>[60x]MRRKVKNTKRHQWRLTHSARSIKRANIMPSNPRGGRRF;>[60x]MKKKMSKLNARVHDFSMFKGNHIPRSKIHIPHKTIRAFNVGEIIPIYQTPVYPGEHIKMDLTSLYRPSTFIVPPMDDLIVDTYAFAVPWRIVWKDLEKFFGENSDSWD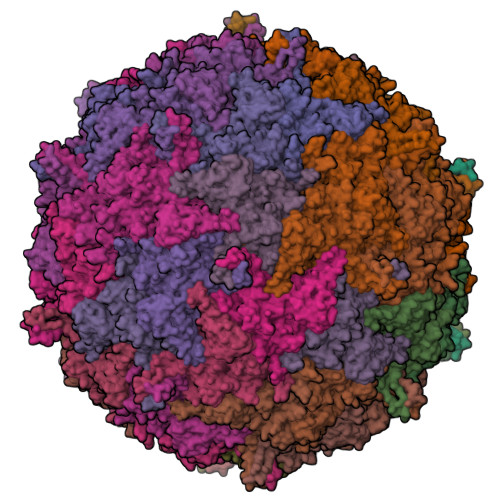VKNAPPVPDIVAPSGGWDYGTLADHFGITPKVPGIRVKSLRFRAYAKIINDWFRDQNLSSECALTLDSSNSQGSNGSNQVTDIQLGGKPYIANKYHDYFTSCLPAPQKGAPTTLNVGGMAPVTTKFRDVPNLSGTPLIFRDNKGRTIKTGQLGIGPVDAGFLVAQNTAQAANGERAIPSNLWADLSNATGISISDLRLAITYQHYKEMDARGGTRYVEFTLNHFGVHTADARLQRSEFLGGHSQSLLVQSVPQTSSTVEKMTPQGNLAAFSETMIQNNYLVNKTFTEHSYIIVLAVVRYKHTYQQGIEADWFRGQDKFDMYDPLLANISEQPVKNREIMVQGNSQDNEIFGFQEAWADLRFKPNSVAGVMRSSHPQSLDYWHFADHYAQLPKLSSEWLKEDYKNVDRTLALKASDNTPQLRVDFMFNTIAEKPMPLYSTPGLRRI>[4x]GHMALSLANYLAADSAAEALRRDVRAGLTATQKSLPPKWFYDAVGSDLFDQITRLPEYYPTRTEAQILRTRSAEIISAAGADTLVELGSGTSEKTRMLLDAMRDAELLRRFIPFDVDAGVLRSAGAAIGAEYPGIEIDAVCGDFEEHLGKIPHVGRRLVVFLGSTIGNL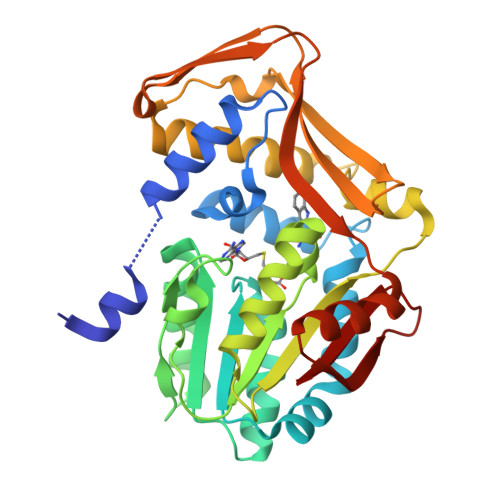TPAPRAEFLSTLADTLQPGDSLLLGTDLVKDTGRLVRAYDDAAGVTAAFNRNVLAVVNRELSADFDLDAFEHVAKWNSDEERIEVWLRARTAQHVRVAALDLEVDFAAGEEMLTAVSCKFRPENVVAELAEAGLRQTHWWTDPAGDFGLSLAVR>MQWSGARALEALLTVAGELRGPPLQLDTGQLLKIAKRGGVTAVEAVHAWRNALTGAPLNLTPEQVVAIASHDGGKQALETVQRLLPVLCQAHGLTPQQVVAIASHDGGKQALETVQRLLPVLCQAHGLTPEQVVAIASHDGGKQALETVQALLPVLCQAHGLTPEQVVAIASNGGGKQALETVQRLLPVLCQAHGLTPQQVVAIASNGGGKQALETVQRLLPVLCQAHGLTPQQVVAIASNGGGKQALETVQRLLPVLCQAHGLTPQQVVAIASNWGGKQALETVQRLLPVLCQAHGLTPQQVVAIASNGGGKQALETVQRLLPVLCQAHGLTPQQVVAIASHDGGKQALETVQRLLPVLCQAHGLTPEQVVAIASNGGGKQALETVQRLLPVLCQAHGLTPEQVVAIASHDGGKQALETVQRLLPVLCQAHGLTPQQVVAIASNGGGRPALESIVAQLSRPDPALAALTNDHLVALACLGGRPALDAVKKLEHHHHHH[2x]

Transcription activator-like (TAL) effectors specifically bind to double stranded (ds) DNA through a central domain of tandem repeats. Each TAL effector (TALE) repeat comprises 33–35 amino acids and recognizes one specific DNA base through a highly variable residue at a fixed position in the repeat. The crystal structures of TAL effector (TALE) proteins bound to their respective target DNAs have revealed that the residue at position 13 is the only one directly involved in DNA base recognition, whereas the 12th residue stabilizes the proper loop conformation. dHax3, an engineered TALE protein, proved to be a useful scaffold for structural characterizations. We then present fifteen crystal structures of engineered dHax3 variants in complex with target DNA molecules, which elucidate the structural basis for the recognition of bases adenine (A) and guanine (G) by reported or uncharacterized TALE codes.

The structural observation suggests that Ile34 may not be a major contributor to the affinity of DNA binding by TALE repeats, consistent with the classification of NI as a “weak” TALE code. It also insinuates that base A may “tolerate” a wide range of amino acids at position 34 of a TALE repeat when there is no steric clash. To test this speculation, we generated dHax3 variants with the 34th residue on repeat 7 substituted with different amino acids. In total, we obtained nine high-quality structures that elucidate the accommodation of base A by Leu, Met, Cys, Pro, Trp, His, Thr, Asn, and Glu at the 34th position. Among these, the hydrophobic residues Leu, Met, Cys, and Pro all adopt conformations that do not clash with base A. As what happens to Ile34, there is no specific coordination found between these hydrophobic residues and base A. Trp, Thr, and His, in spite of the presence of polar groups, do not form H-bond with base A. They also appear to adopt conformations that simply avoid steric clash. These residues may all represent weak code, if they are used for base recognition.> MADPSLHHEAQPLKFIAVDYCPESCTHSPESSTITLTFDHRGGSRWRSTTRFQYGTFSSLIQCPK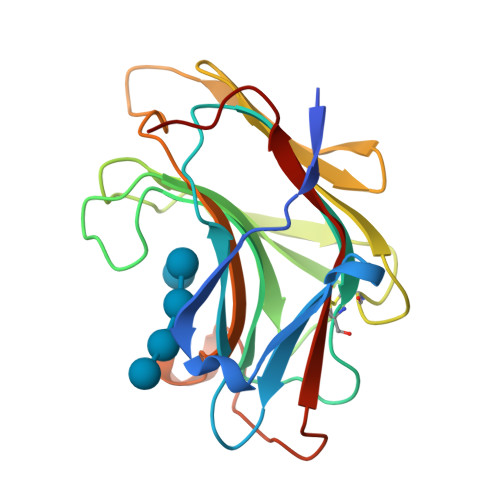GNTSGLNFNIYLSSLEGDKSQDAIDFEFLGKDKRIVQTNYYTAGTGNREAIHDLGFDCSDGFHEYVIKWGPDLIQWLIDGKVIRSVRADGEGFPQKPMFLYASVWDASYIDEGRWTGPYVGCDAPYICLYKNVNVPVGTAVE> KHTLPDLPFDYADLEPVISHEIMQLHHQKQHATYVNNLNQIEEKLHEAVSKGNLKEAIALQPALKFNGGGHINHSIFWTNLAKDGGEPSKELMDTIKRDFGSLDNLQKRLSDITIAVQGSGWGWLGYCKKDKILKIATCANQDPLEGMVPLFGIDVWEHAYYLQYKNVR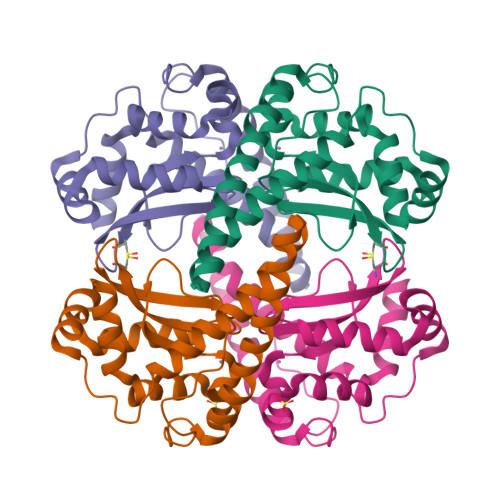PDYVHAIWKIANWKNISERFANARQ;> MKHTLPDLPFDYADLEPVISHEIMQLHHQKQHATYVNNLNQIEEKLHEAVSKGNLKEAIALQPALKFNGGGHINHSIFWTNLAKDGGEPSKELMDTIKRDFGSLDNLQKRLSDITIAVQGSGWGWLGYCKKDKILKIATCANQDPLEGMVPLFGIDVWEHAYYLQYKNVRPDYVHAIWKIANWKNISERFANARQ> MALAKRIDAALIMKDGRVVKGSNFENLRDSGDPVELGKFYSEIGIDELSFWDITASVEKRKTMLELVEKVAEQID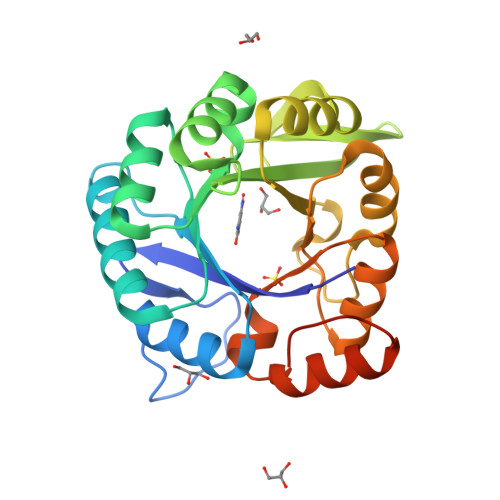IPITVGGGIHDFETASELILRGADKVEFNTAAVENPSLITQIAQTFGSQAVVVYIAAKRVDGEFMVFTYSGTKNTGILLRDWVVEVEKRGAGEIVLGSIDRLGTKSGYDTEMIRFVRPLTTLPIIAHRGAGKMEHFLEAFLAGADAAKADSVFHSREIDVRELKEYLKKHGVNVRLEGLGSLEHHHHHH>[8x]GVALGATRVIYPAGQKQVQLAVTNNDENSTYLIQSWVENADGVKDGRFIVTPPLFAMKGKKENTLRILDATNNQLPQDRESLFWMNVKAIPSMDKSKLTENTLQLAIISRIKLYYRPAKLALPPDQAAEKLRFRRSANSLTLINPTP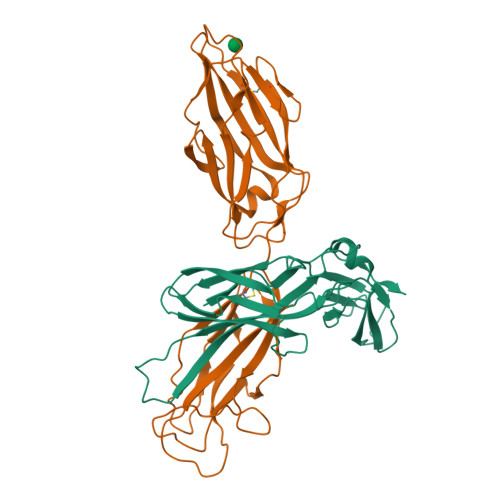YYLTVTELNAGTRVLENALVPPMGESTVKLPSDAGSNITYRTINDYGALTPKMTGVME;>FACKTANGTAIPIGGGSANVYVNLAPVVNVGQNLVVDLSTQIFCHNDYPETITDYVTLQRGSAYGGVLSNFSGTVKYSGSSYPFPTTSETPRVVYNSRTDKPWPVALYLTPVSSAGGVAIKAGSLIAVLILRQTNNYNSDDFQFVWNIYANNDVVVPTGGCDVSARDVTVTLPDYPGSVPIPLTVYCAKSQNLGYYLSGTTADAGNSIFTNTASFSPAQGVGVQLTRNGTIIPANNTVSLGAVGTSAVSLGLTANYARTGGQVTAGNVQSIIGVTFVYQ[8x]In its active tetradecameric conformation, ClpP forms the central proteolytic compartment of a larger AAA+ protease machine. Two rings of seven ClpP monomers stack and interact to form a secluded barrel‐shaped tetradecamer harbouring the 14 catalytic sites. Small entrance pores at the top and bottom of the barrel restrict access of proteins and allow isolated ClpP to degrade small peptides only. For protein degradation, Clp‐ATPases are required (in Firmicutes ClpX, ClpC, and ClpE) to unfold designated substrates and thread them through the entrance pores.

In order to gain further insight into the interaction of ADEP with ClpP from S. aureus and thereby support our functional analyses of the mutated S. aureus ClpP proteins, we generated and solved the corresponding co‐crystal structure in conjunction with the apo‐protein at resolutions of 2.2 Å and 1.9 Å, respectively. In the apo structure of S. aureus ClpP presented here, two distinct conformations can be differentiated, like in a previous crystal structure of ClpP. Five out of seven subunits display a well‐defined upwards pointing β‐hairpin loop and downwards facing N termini. In contrast, in the remaining two, a structural inversion of the first nineteen amino acids can be observed. This inversion leads to the loss of the structured hairpin and the respective N termini are facing upwards with a slight tilt towards the barrel rotation axis. The residues E9 to D19 form a loop that extends into the axial channel and, in conjunction with the terminal residues M1 to V7, facilitate pore closure. In our apo‐ClpP structure, where two out of seven subunits are in this disordered state, the pore is effectively closed. An overlay of the D27 moieties of all ClpP subunits within one apo‐ClpP ring shows a stable conformation in suitable H‐bond distance to R23, while upon insertion of the hydrophobic ADEP tail region this order is disturbed. In apo‐ClpP residues 1–19 are highly flexible, dynamically alternating between two states. The first state is characterised by an ordered upwards‐pointing β‐hairpin, stabilised by a network of electrostatic interactions between E9, R23 and D27.

>MNLIPTVIETTNRGERAYDIYSRLLKDRIIMLGSQIDDNVANSIVSQLLFLQAQDSEKDIYLYINSPGGSVTAGFAIYDTIQHIKPDVQTICIGMAASMGSFLLAAGAKGKRFALPNAEVMIHQPLGGAQGQATEIEIAANHILKTREKLNRILSERTGQSIEKIQKDTDRDNFLTAEEAKEYGLIDEVMVPETKWSHPQFEK[14x]>GSHMDEGKITVFAACSLTNAMQDIATQFKKEKGVDVVSSFASSSTLARQIEAGAPADLFISADQKWMDYAVDKKAIDTATRQTLLGNSLVVVAPKASVQKDFTIDSKTNWTSLLNGGRLAVGDPEHVPAGIY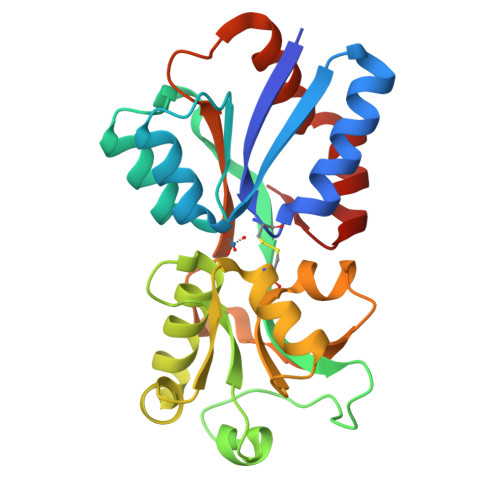AKEALQKLGAWDTLSPKLAPAEDVCGALALVERNEAPLGIVYGSDAVASKGVKVVATFPEDSHKKVEYPVAVVEGHNNATVKAFYDYLKGPQAAEIFKRYGFTIK[3x]>[4x]MSFMDQIPGGGNYPKLPVECLPNFPIQPSLTFRGRNDSHKLKNFISEIMLNMSMISWPNDASRIVYCRRHLLNPAAQWANDFVQEQGILEITFDTFIQGLYQHFYKPPDINKIFNAITQLSEAKLGIERLNQRFRKIWDRMPPDFMTEKAAIMTYTRLLTKETYNIVRMHKPETLKDAMEEAYQTTALTERFFPGFELDADGDTIIGATTHLQEEYDSDYDSEDNLTQNGYVHTVRTRRSYNKPMSNHRNRRNNNPSREECIKNRLCFYCKKEGHRLNECRARKAVLTDLELESKDQQTPFIKTLPIVHYIAIPEMDNTAEKTIKIQNTKVKTLFDSGSPTSFIRRDIVELLKYEIYETPPLRFRGFVATKSAVTSEAVTIDLKINDLHITLAAYILDNMDYQLLIGNPILRRYPKILHTVLNTRESPDSLKPKTYRSETVNNVRTYSAGNRGNPRNIKLSFAPTILEATDPKSAGNRGDSRTKTLSLATTTPAAIDPLTTLDNPGSTQSTFAQFPIPEEASILEEDGKYSNVVSTIQSVEPNATDHSNKDTFCTLPVWLQQKYREIIRNDLPPRPADINNIPVKHDIEIKPGARLPRLQPYHVTEKNEQEINKIVQKLLDNKFIVPSKSPCSSPVVLVPKKDGTFRLCVDYRTLNKATISDPFPLPRIDNLLSRIGNAQIFTTLDLHSGYHQIPMEPKDRYKTAFVTPSGKYEYTVMPFGLVNAPSTFARYMADTFRDLRFVNVYLDDILIFSESPEEHWKHLDTVLERLKNENLIVKKKKCKFASEETEFLGYSIGIQKIAPLQHKCAAIRDFPTPKTVKQAQR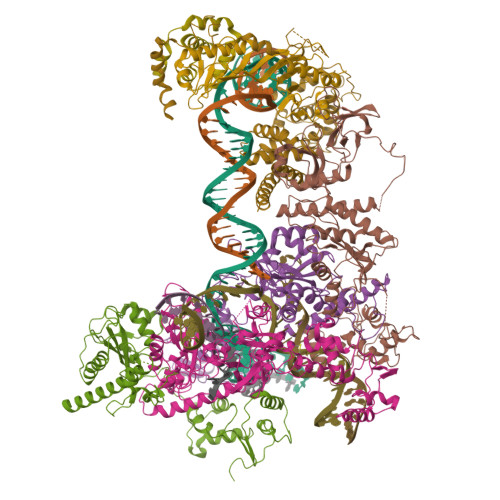FLGMINYYRRFIPNCSKIAQPIQLFICDKSQWTEKQDKAIDKLKDALCNSPVLVPFNNKANYRLTTDASKDGIGAVLEEVDNKNKLVGVVGYFSKSLESAQKNYPAGELELLGIIKALHHFRYMLHGKHFTLRTDHISLLSLQNKNEPARRVQRWLDDLATYDFTLEYLAGPKNVVADAISRAVYTITPETSRPIDTESWKSYYKSDPLCSAVLIHMKELTQHNVTPEDMSAFRSYQKKLELSETFRKNYSLEDEMIYYQDRLVVPIKQQNAVMRLYHDHTLFGGHFGVTVTLAKISPIYYWPKLQHSIIQYIRTCVQCQLIKSHRPRLHGLLQPLPIAEGRWLDISMDFVTGLPPTSNNLNMILVVVDRFSKRAHFIATRKTLDATQLIDLLFRYIFSYHGFPRTITSDRDVRMTADKYQELTKRLGIKSTMSSANHPQTDGQSERTIQTLNRLLRAYASTNIQNWHVYLPQIEFVYNSTPTRTLGKSPFEIDLGYLPNTPAIKSDDEVNARSFTAVELAKHLKALTIQTKEQLEHAQIEMETNNNQRRKPLLLNIGDHVLVHRDAYFKKGAYMKVQQIYVGPFRVVKKINDNAYELDLNSHKKKHRVINVQFLKKFVYRPDAYPKNKPISSTERIKRAHEVTALIGIDTTHKTYLCHMQDVDPTLSVEYSEAEFCQIPERTRRSILANFRQLYETQDNPEREEDVVSQNEICQYDNTSP;> MSSIVNKSGTRFAPKVRQRRAATGGTPTPKPRTPQLFIPESKEIEEDNSDNDKGVDENETAIVEKPSLVGERSLEGFTLTGTNGHDNEIGDEGPIDASTQNPKADVIEDNVTLKPAPLQTHRDQKVPRSSRLASLSKDNESRPSFKPSFLDSSSNSNGTARRLSTISNKLPKKIRLGSITENDMNLKTFKRHRVLGKPSSAKKPAGAHRISIVSKISPPTAMTDSLDRNEFSSETSTSREADENENYVISKVKDIPKKVRDGESAKYFIDEENFTMAELCKPNFPIGQISENFEKSKMAKKAKLEKRRHLRELRMRARQEFKPLHSLTKEEQEEEEEKRKEERDKLLNADIPESDRKAHTAIQLKLNPDGTMAIDEETMVVDRHKNASIENEYKEKVDENPFANLYNYGSYGRGSYTDPWTVEEMIKFYKALSMWGTDFNLISQLYPYRSRKQVKAKFVNEEKKRPILIELALRSKLPPNFDEYCCEIKKNIGTVADFNEKLIELQNEHKHHMKEIEEAKNTAKEEDQTAQRLNDANLNKKGSGGIMTNDLKVYRKTEVVLGTIDDLKRKKLKERNNDDNEDNEGSEEEPEIDQ;> MADEERLKEFKEANKIVFDPNTRQVWENQNRDGTKPATTFQSEEDIKRAAPESEKDTSATSGIVPTLQNIVATVTLGCRLDLKTVALHARNAEYNPKRFAAVIMRIREPKTTALIFASGKMVVTGAKSEDDSKLASRKYARIIQKIGFAAKFTDFKIQNIVGSCDVKFPIRLEGLAFSHGTFSSYEPELFPGLIYRMVKPKIVLLIFVSGKIVLTGAKQREEIYQAFEAIYPVLSEFRKM;> MPVCKNCHGTEFERDLSNANNDLVCKACGVVSEDNPIVSEVTFGETSAGAAVVQGSFIGAGQSHAAFGGSSALESREATLNNARRKLRAVSYALHIPEYITDAAFQWYKLALANNFVQGRRSQNVIASCLYVACRKEKTHHMLIDFSSRLQVSVYSIGATFLKMVKKLHITELPLADPSLFIQHFAEKLDLADKKIKVVKDAVKLAQRMSKDWMFEGRRPAGIAGACILLACRMNNLRRTHTEIVAVSHVAEETLQQRLNEFKNTKAAKLSVQKFRENDVEDGEARPPSFVKNRKKERKIKDSLDKEEMFQTSEEALNKNPILTQVLGEQELSSKEVLFYLKQFSERRARVVERIKATNGIDGENIYHEGSENETRKRKLSEVSIQNEHVEGEDKETEGTEEKVKKVKTKTSEEKKENESGHFQDAIDGYSLETDPYCPRNLHLLPTTDTYLSKVSDDPDNLEDVDDEELNAHLLNEEASKLKERIWIGLNADFLLEQESKRLKQEADIATGNTSVKKKRTRRRNNTRSDEPTKTVDAAAAIGLMSDLQDKSGLHAALKAAEESGDFTTADSVKNMLQKASFSKKINYDAIDGLFR>MPVFDEPVYTVNVLENSPINTLVIDLNATDPDEGTNGEVVYSFINFVSNLTKQMFKIDPKTGVITVNGVLDHEELHIHEIDVQAKDLGPNSIPAHCKVIVNVIDINDNAPEIKLLSENSEMVEVSENAPLGYVIALVRVSDNDSGANGKVQCRLQGNVPFRLNEFESFSTLLVDGRLDREQRDM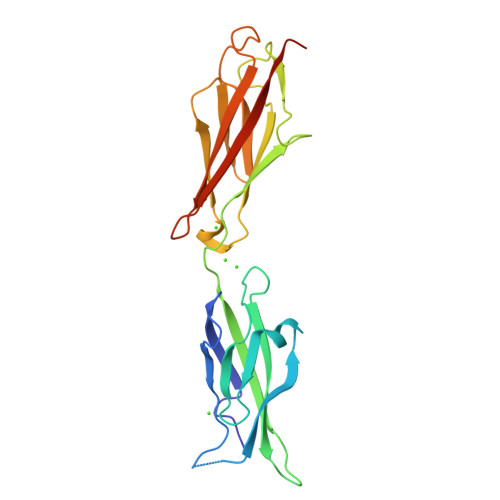YNLTILAEDSGYPPLRSSKSFAVKVTDLEHHHHHH[4x]>[2x]MTMAGQTINDRLLAARHSLAGQGLAKSVCKATTEECIGPKKKHLDYLVHCANEPNVSIPHLANLLIERSQNANWVVVYKSLITTHHLMAYGNERFMQYLASSNSTFNLSSFLDKGTVQDGGMGVPGGRMGYDMSPFIRRYAKYLNEKSLSYRAMAFDFCKVKRGKEEGSLRSMNAEKLLKTLPVLQAQLDALLEFDCQSN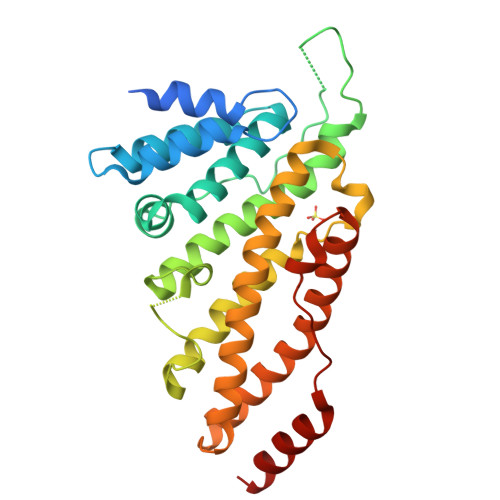DLSNGVINMSFMLLFRDLIRLFACYNDGIINLLEKYFDMNKKHARDALDLYKKFLVRMDRVGEFLKVAENVGIDKGDIPDLTKAPSSLLDALEQHLATL>[4x]GSAAQGTVRKAGALAVKNFLVHKKNKKVESATRRKWKHYWVSLKGCTLFFYESDGRSGIDHNSIPKHAVWVENSIVQAVPEHPKKDFVFCLSNSLGDAFLFQTTSQTELENWITAIHSACATAVARHHHKEDTLRLLKSEIKKLEQKIDMD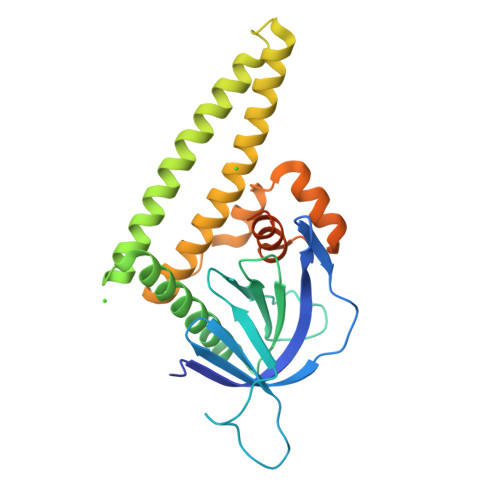EKLKKMGELQLSSVTDSKAAATILDQIFVWEQNLEQFQMDLFRFRCYLASLQGGELPNPKRLLAFASRPTKVAMGRLGIFSVSSFHALVAARTGETGVRRRTQAMSRSASKRRSRFSSLWGLDTT>[2x]GSKNTSGDLSQKQALQLALSAREHFWNTMSGHNPKVKKAVCPSGTFEYQNLQYVYMCSDLGTKAKAVNYLTPIFTKTAIEKGFKDYHFTVSKGKLAVPIGDGDNLLNWKKSTAKLISKKGSTITYEFTVPTLDGSPSAKRKVTFVKENKKWKVNQFDAVI;>GSQSIKVKKGDTLWDLSRKYDTTISKI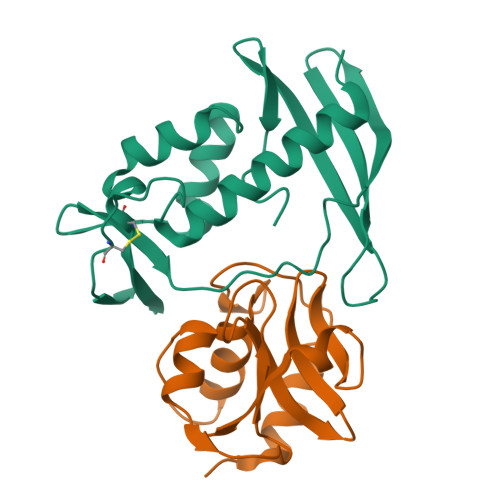KSENHLRSDIIYVGQTLSINGKSTSSKSSSSSSSSSTYKVKSGDSLWKISKKYGMTINELKKLNGLKSDLLRVGQVLKLKGSTSSSSSSSSKVSSSSTSTYKVKSGDSLSKIASKYGTTVSKLKSLNGLKSDVIYVNQVLKVKGTSTSSSKPASSSSSSSSKTSSTSLNVSKLVSDAKALVGTPYKWGGTTTSGFDCSGFIWYVLNKQTSVGRTSTAGYWSSMKSIASPSVGDFVFFTTYKSGPSHMGIYIGNNSFIHAGSDGVQISSLNNSYWKPRYLGAKRF[2x]>[4x]GSHMTQDCSFQHSPISSDFAVKIRELSDYLLQDYPVTVASNLQDEELCGGLWRLVLAQRWMERLKTVAGSKMQGLLERVNTEIHFVTKCAFQPPPSCLRFVQTNISRLLQETSEQLVALKPWITRQNFSRCLELQCQP;>ETGNQDLPVIKCVLINHKNNDSSVGKSSSYPMVSESPEDLGCALRPQSSGTVYEAAAVEVDVSASITLQVLVDAPGNISCLWVFKHSSLNCQPHFDLQNRGVVSMVILKMTETQAGEYLLFIQSEATNYTILFTVSIRNTLLYTLRRPYFRKMENQDALVCISESVPEPIVEWVLCDSQGESCKEESPAVVKKEEKVLHELFGTDIRCCARNELGRECTRLFTIDLNQTPQTTLPQLFLKV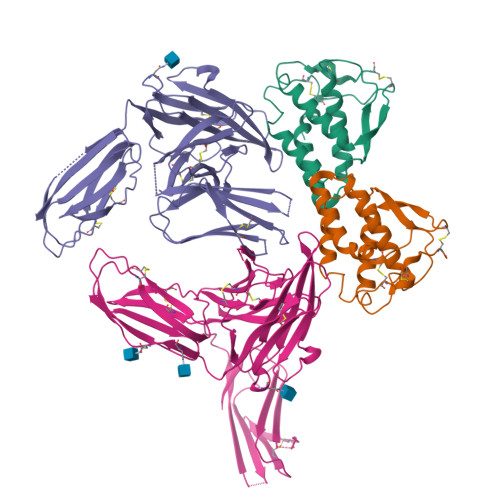GEPLWIRCKAVHVNHGFGLTWELENKALEEGNYFEMSTYSTNRTMIRILFAFVSSVARNDTGYYTCSSSKHPSQSALVTIVEKGFINATNSSEDYEIDQYEEFCFSVRFKAYPQIRCTWTFSRKSFPCEQKGLDNGYSISKFCNHKHQPGEYIFHAENDDAQFTKMFTLNIRSGTKHHHHHH[4x]>VFSITTLRDWTPDPGSIICWHASPTAKAKARQAPISEVPPSYQQAQHLRRYRDHVARGLDMSRLMIFTWDLPGRCNIRAMNYAINAHLRRHDTYHSWFEFDNAEHIVRHTIADPADIEVVQAEHQNMTSAELRHHIATPQPLQWDCFLFGIIQSDDHFTFYASIAHLCVDPMIVGVLFIEIHMMYSALVGGDPPIELPPAGRYDDHCVRQYADTAALTLDSARVRRWVEFAANNDGTLPHFPLPLGDLSVPHTGKLLTETLMDEQQGERFEAACVAAGARFSGGVFACAALAERELTNCETFDVVTTTDTRRTPTELRTTGWFTGLVPITVPVASGLFDSAARVAQISFDSGKDLATVPFDR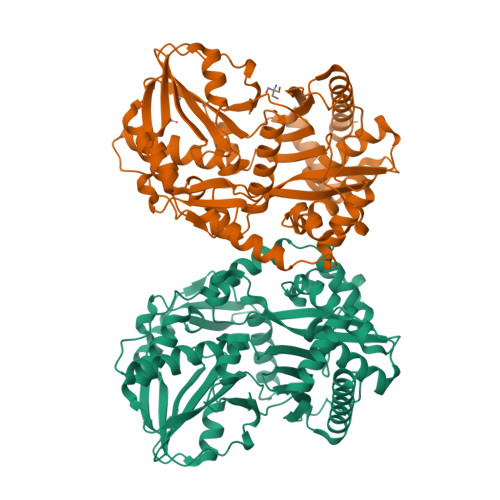VLELARPETGLRPPRPGNFVMSFLDASIAPLSTVANSDLNFRIYDEGRVSHQVSMWVNRYQHQTTVTVLFPDNPIASESVANYIAAMKSIYIRTADGTLATLKPGT[2x]>[4x]MEAVPRMPMIWLDLKEAGDFHFQPAVKKFVLKNYGENPEAYNEELKKLELLRQNAVRVPRDFEGCSVLRKYLGQLHYLQSRVPMGSGQEAAVPVTWTEIFSGKSVAHEDIKYEQACILYNLGALHSMLGAMDKRVSEEGMKVSCTHFQCAAGAFAYLREHFPQAYSVDMSRQILTLNVNLMLGQAQECLLEKSMLDNRKSFLVARISAQVVDYYKEACRALENPDTASLLGRIQKDWKKLVQMKIYYFAAVAHLHMGKQAEEQQKFGERVAYFQSALDKLNEAIKLAKGQPDTVQDALRFTMDVIGGKYNSAKKDNDFIYHEAVPALDTLQPVKGAPLVKPLPVNPTDPAVTGPDIFAKLV;>QRAEEEDDDIKQLAAWAT[4x]

His domain protein tyrosine phosphatase (HD-PTP/PTPN23) is a tumor suppressor that regulates mitogenic receptor downregulation, endocytic recycling, and cell migration (Chen et al., 2012, Doyotte et al., 2008, Kharitidi et al., 2015, Lee et al., 2007, Ma et al., 2015, Manteghi et al., 2016). A central feature of HD-PTP function is the ability of its Bro1 domain to recruit CHMP4, the major subunit of the ESCRT-III membrane remodeling protein complex (Doyotte et al., 2008, Ichioka et al., 2007, Parkinson et al., 2015). Crystallographic structures of the HD-PTPBro1 domain in complex with the relevant binding regions of SARA, endofin, and all three human CHMP4 isoforms reveal that SARA and endofin binding is similar to that of CHMP4 at the conserved site, but critically extends into a neighboring specific pocket unique to HD-PTP. Altogether, this study identifies the Bro1 domain of HD-PTP as a highly selective interaction hub that coordinates recruitment of endosomal signaling adaptors versus MVB sorting and receptor degradation.

Next, peptides designed from the C-terminal 18–20 residues of CHMP4A, CHMP4B, and CHMP4C were evaluated for binding to HD-PTPBro1. Interestingly, CHMP4 peptides showed much lower affinity to HD-PTPBro1 compared with the SARA/endofin peptides, with KD values of 132 ± 7 μM for CHMP4A, 85 ± 2 μM for CHMP4B, and 89 ± 1 μM for CHMP4C. For the CHMP4 peptides only 11 residues are clearly visible in the electron density maps, whereas 20 residues are visible for the SARA and endofin peptides. All three CHMP4 peptides bind in the same way across helices H5, H6, and H7 of HD-PTPBro1, and form similar van der Waals contacts with a number of conserved residues, including the critical L202/I206 pair. Additional contacts occur with hydrophobic residues at the proline-rich C-terminal region of HD-PTPBro1 (see Table 2 for a list of all interactions). The main CHMP4 anchoring residues are a Leu and a Trp present in all three isoforms (L217 and W220 in CHMP4A and CHMP4B, L228/W231 in CHMP4C), which contact HD-PTPBro1 residues L189, L202, and I206 from two hydrophobic pockets between H5 and H6 and H6 and H7. The mode of binding of CHMP4 peptides to HD-PTPBro1 is similar to that reported for the complexes of CHMP4 peptides with Alix or Brox Bro1 domains (McCullough et al., 2008, Mu et al., 2012). Thus, binding of CHMP4A/B/C to HD-PTPBro1 requires rearrangement of these side chains to accommodate the critical CHMP4 Leu and Trp residues. Overall, the SARA/endofin peptides form an extensive binding interface that encompasses both the CHMP4 site and the S site, resulting in accessible buried surface in HD-PTPBro1 ranging from 762 to 780 Å2, compared with 468 to 473 Å2 for the CHMP4 peptides.> QLDKKYKHAGDFGISDTKKNRETLTKFRDAIEEHLSDKDTVEKGTYRREKGSKVYFNPNTMNVVIIKSNGEFLSGWKINPDADNGRIYLETGEL;> NKMAMIDLAKLFLASKITAIEFSERICVERRRLYGVKDLSPNILNCGEELFMAAERFEPDADRANYEIDDNGLKVEVRSILEKFK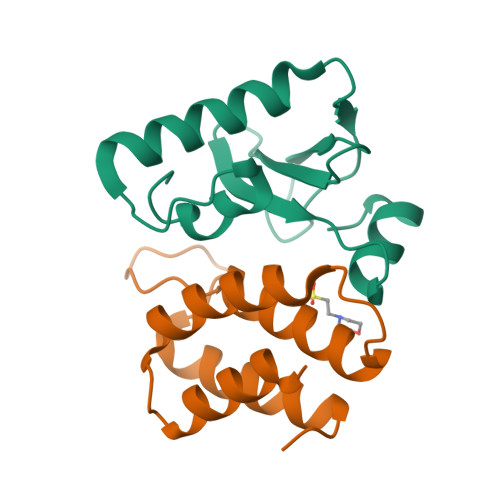LHHHHH>KHDCVICFENEVIAALVPCGHNLFCMECANKICEKRTPSCPVCQT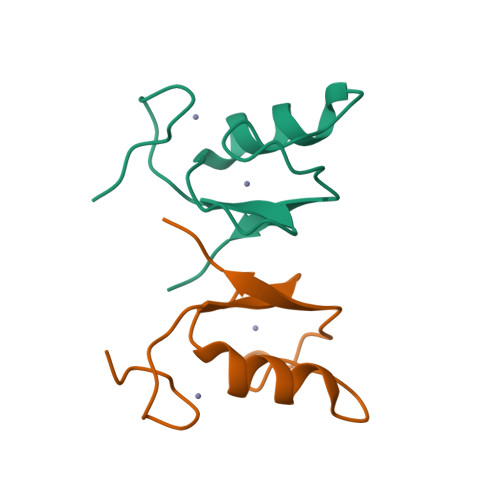AVTQAIQIHS[8x]>[2x]MANAYKQAGVDIEAGYEAVSRMKKHVQTTMRKEVLGGLGGFGGMFDLSKFALEEPVLVSGTDGVGTKLMLAFMADKHDTIGIDAVAMCVNDIVVQGAEPLFFLDYIACGKAEPSKIENIVKGISEGCRQAGCALIGGETAEMPGMYSTEEYDLAGFTVGIVDKKKIVTGEKIEAGHVLIGLASSGIHSNGYSLVRKVLLEDGELSLDRIYGRLELPLGEELLKPTKIYVK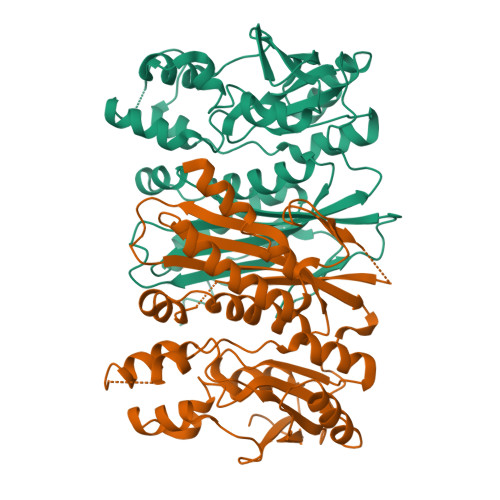PILELLKNHEVYGMAHITGGGFIENIPRMLPEGIGAEIELGSWKIQPIFSLLQEVGKLEEKEMFNIFNMGIGMVVAVKEEDAKDIVRLLEEQGETARIIGRTVQGAGVTFNGGKAL> MPARALLPRRMGHRTLASTPALWASIPCPRSELRLDLVLPSGQSFRWREQSPAHWSGVLADQVWTLTQTEEQLHCTVYRGDKSQASRPTPDELEAVRKYFQLDVTLAQLYHHWGSVDSHFQEVAQKFQGVRLLRQDPIECLFSFICSSNNNIARITGMVERLCQAFGPRLIQLDDVTYHGFPSLQALAGPEVEAHLRKLGLGYRARYVSASARAILEEQGGLAWLQQLRESSYEEAHKALCILPGVGTKVADCICLMALDKPQAVPVDVHMWHIAQRDYSWHPTTSQAKGP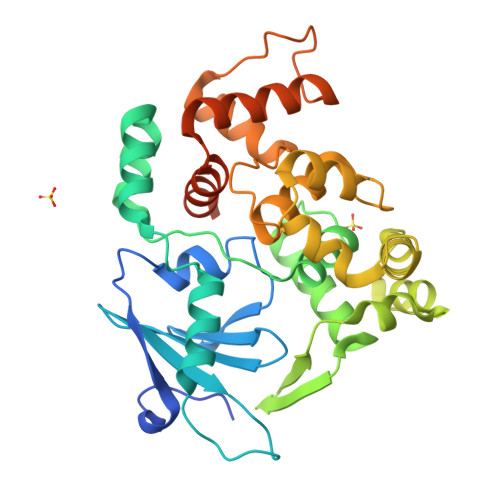SPQTNKELGNFFRSLWGPYAGWAQAVLFSADLRQSRHAQEPPAKRRKGSKGPEG>[2x]MSENSIRLTQYSHGAGCGCKISPKVLETILHSEQAKFVDPNLLVGNE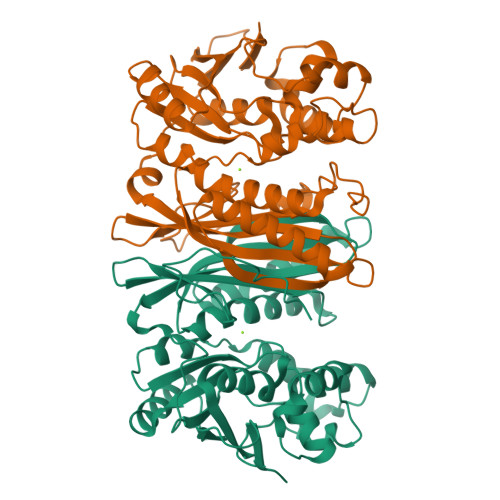TRDDAAVYDLGNGTSVISTTDFFMPIVDNPFDFGRIAATNAISDIFAMGGKPIMAIAILGWPINKLSPEIAREVTEGGRYACRQAGIALAGGHSIDAPEPIFGLAVTGIVPTERVKKNSTAQAGCKLFLTKPLGIGVLTTAEKKSLLKPEHQGLATEVMCRMNIAGASFANIEGVKAMTDVTGFGLLGHLSEMCQGAGVQARVDYEAIPKLPGVEEYIKLGAVPGGTERNFASYGHLMGEMPREVRDLLCDPQTSGGLLLAVMPEAENEVKATAAEFGIELTAIGELVPARGGRAMVEIR> GSHMGGELKTVTLSKMKQSLGISISGGIESKVQPMVKIEKIFPGGAAFLSGALQAGFELVAVDGENLEQVTHQRAVDTIRRAYRNKAREPMELVVRVPGPSGSAYGSVKAYTNFDAERDALNIETAIKTKGVDEVTIVNILTNRSNEQRQDIAFAYQRRTKKELASALKSALSGHLETVILGLLKTPAQYDASELKASMKGLGTDEDSLIEIICSRTNQELQEINRVYKEMYKTDLEKDIISDTSGDFRKLMVALAK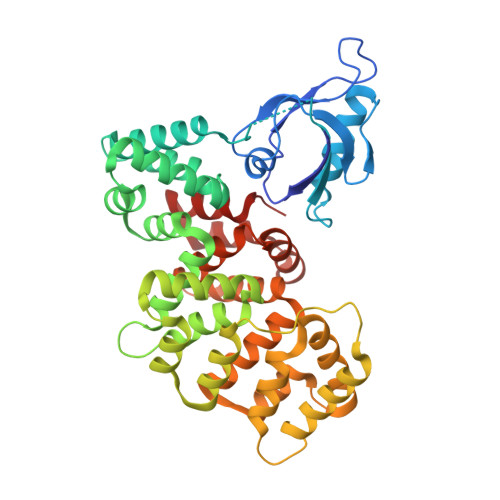GRRAEDGSVIDYELIDQDARDLYDAGVKRKGTDVPKWISIMTERSVPHLQKVFDRYKSYSPYDMLESIRKEVKGDLENAFLNLVQCIQNKPLYFADRLYDSMKGKGTRDKVLIRIMVSRSEVDMLKIRSEFKRKYGKSLYYYIQQDTKGDYQKALLYLCGGDD N-[2-(4-{4-[2-amino-4-(difluoromethyl)pyrimidin-5-yl]-6-(morpholin-4-yl)-1,3,5-triazin-2-yl}piperazin-1-yl)-2-oxoethyl]-1-(prop-2-enoyl)piperidine-4-carboxamide | 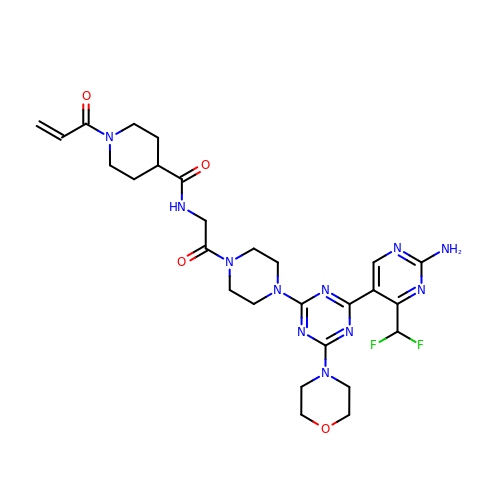C27 H35 F2 N11 O4 | YAPSKJOBRAWBJI-UHFFFAOYSA-N>[2x]LDKLHVTSTRPQYVRIKNWGSGEILHDTLHHKATSDFTCKSKSCLGSIMNPKSLTRGPRDKPTPLEELLPHAIEFINQYYGSFKEAKIEEHLARLEAV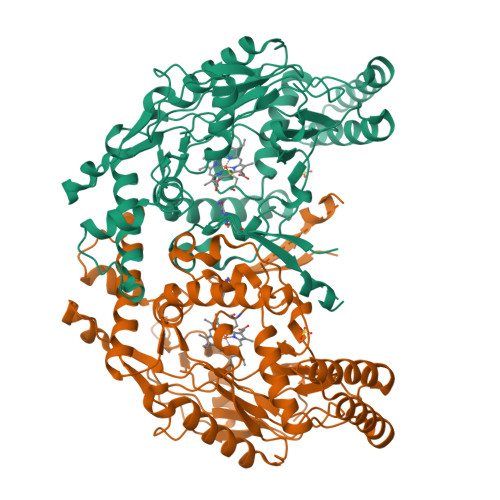TKEIETTGTYQLTLDELIFATKMAHRNAPRCIGRIQWSNLQVFDARNCSTAQEMFQHICRHILYATNNGNIRSAITVFPQRSDGKHDFRLWNSQLIRYAGYQMPDGTIRGDAATLEFTQLCIDLGWKPRYGRFDVLPLVLQADGQDPEVFEIPPDLVLEVTMEHPKYEWFQELGLKWYALPAVANMLLEVGGLEFPACPFNGWYMGTEIGVRDFCDTQRYNILEEVGRRMGLETHTLASLWKDRAVTEINVAVLHSFQKQNVTIMDHHTASESFMKHMQNEYRARGGCPADWIWLVPPVSGSITPVFHQEMLNYVLSPFYYYQIEPWKTHIWQ> GSVYPKELTQVFEHYINNNLFDIDSLVKFIEELGYNLEDLATLCLAHLLGYKKLEEPLKREDFLSTWFMQGCSTISDMQECIKTLDVKLHEDLQYFTQIYNYAFNLILDPNRKDIDTDEG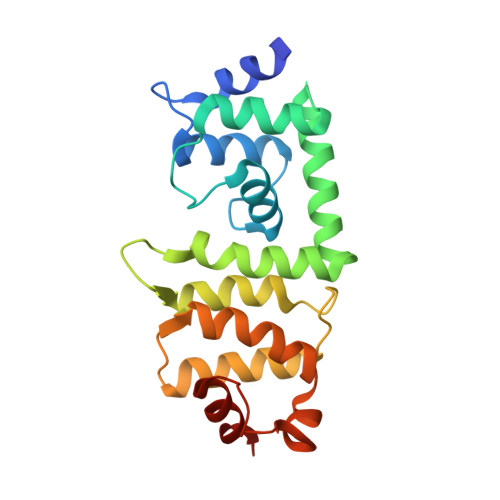IQYWKLFFQPEYPVRMEPDLLEAWFRFLRDEGKTTISKDTWRMLLLFFKRYPTIQKIISDYDETAAWPFIIDEFYECLQDQQ>HHHSSGLTPRGSQMKKIAFGCDHVGFILKHEIVAHLV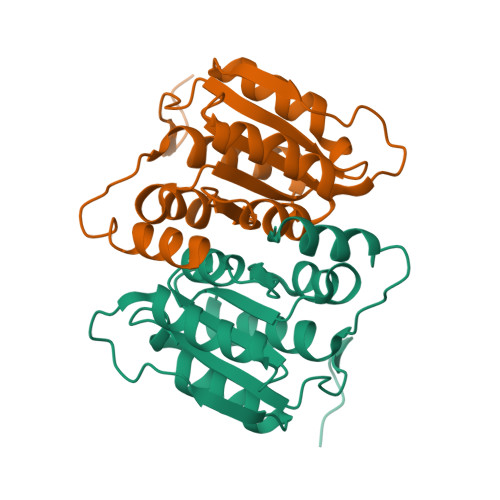ERGVEVIDKGTWSSERTDYPHYASQVALAVAGGEVDGGILICGTGVGISIAANKFAGIRAVVCSEPYSAQLSRQHNDTNVLAFGSRVVGLELAKMIVDAWLGAQYEGGRHQQRVEAITAIEQRRN[4x]> MADDWKPQILAIICNWCSYAGADLAGGARIQYPPTVRAIRVMCTGRVDMLFILKAFVEGADGVLVSGCHFGDCHYLEGNYKAAKRMFMIKNLLRNIGLDDRRFRMTFVSASEGAKWGMVMEDVTNTIKELGPSPI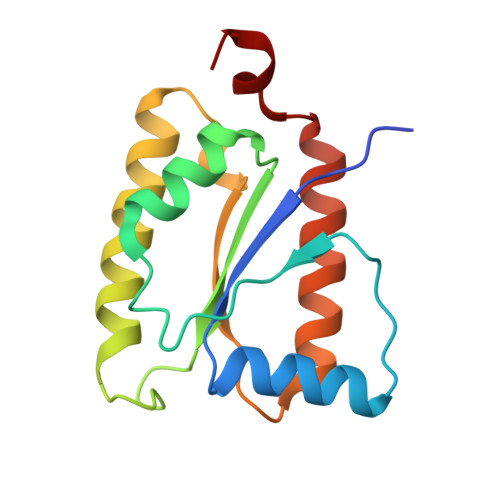KEFKK> GSHMASMSKDEVKREAKDTDGNPEIKGERRRLHSEIQSGSLANNIKKSTVIVKAPTHIAICLYYKLGETPLPLVIETGK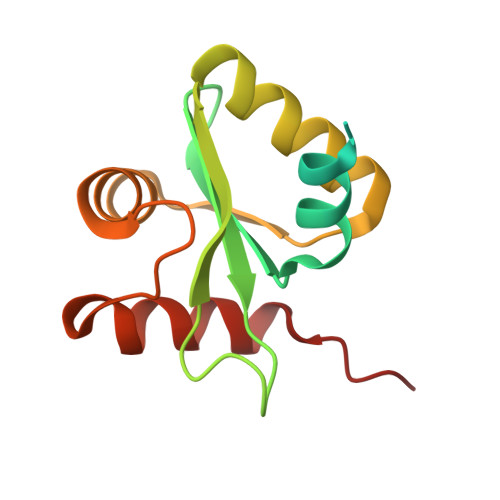DAKALQIIKLAELYDIPVIEDIPLARSLYKNIHKGQYITEDFFEPVAQLIRIAIDLDY>[2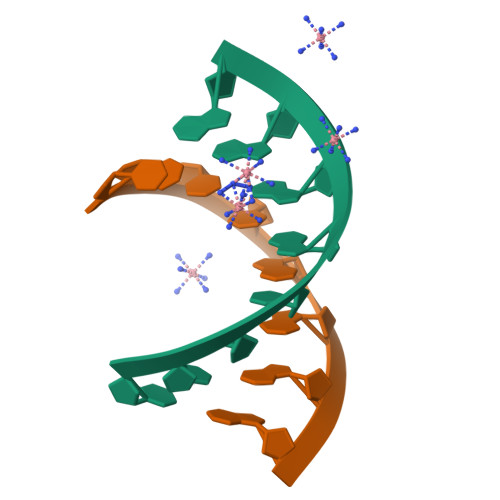x]CCCCXGGG> KAGSAAAPFTKPFAVYKNVKFYLGDISHLVNCVSFDFVVNAANENLLHGGGVARAIDILTEGQLQSLS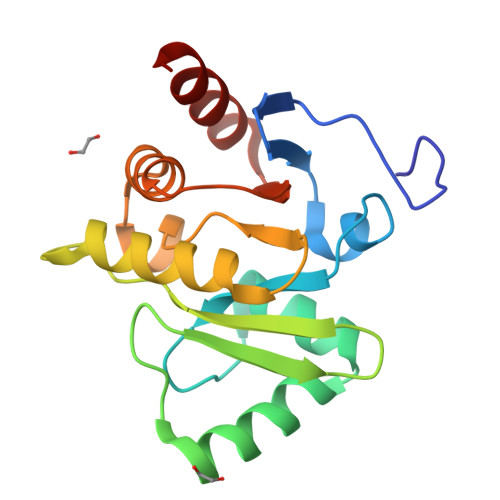KDYISSNGPLKVGAGVMLECEKFNVFNVVGPRTGKHEHSLLVEAYNSILFENGIPLMPLLSCGIFGVRIENSLKALFSCDINKPLQVFVYSSNEEQAVLKFLDGLD> GTSYENSLLVKQSGSLPLSSLTHVLRSLTPNARGIFRLLIKYQLDNQDNPSYIGLSFQDFYQQCREAFLVNSDLTLRAQLTEFRDHKLIRTKKGTDGVEYLLIPVDNGT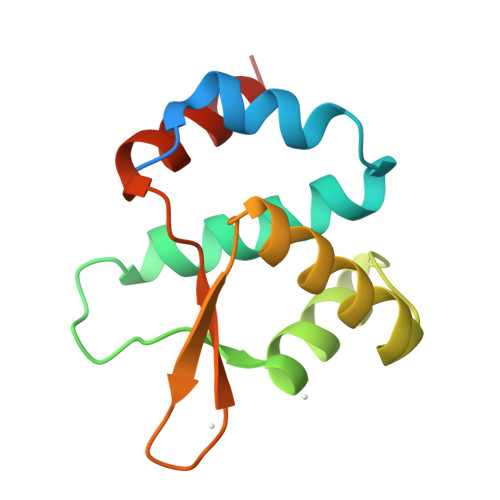LTDFLEKEEEEA> PAKKPLTKIVSHLLVAEPDKLYAMPPPGMPEGDIKALTTLCDLADRELVVIIGWAKHIPGFSSLSLGDQMSLLQSAWMEILILGIVYRSLPYDDKLVYAEDYIMDEEHSRLAGLLELYRAILQLVRRYKKLKVEKEEFVTLKALALANSDSMYIEDLEAVQKLQDLLHEALQDYELSQRHEEPWRTGKL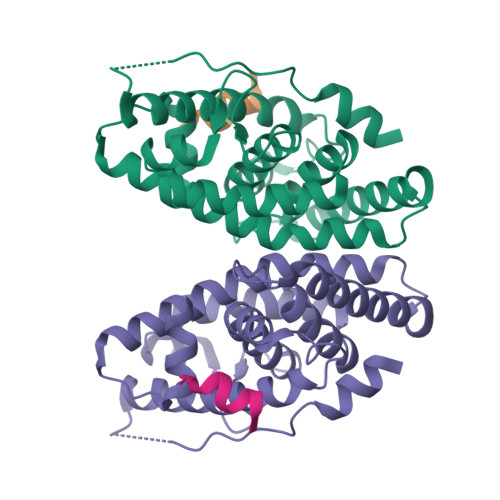LLTLPLLRQTAAKAVQHFYSVKLQGKVPMHKLFLEMLEAK;> ASELLKYLTT(3alpha,8alpha)-3,17-dihydroxypregn-5-en-20-one | C21 H32 O3 | 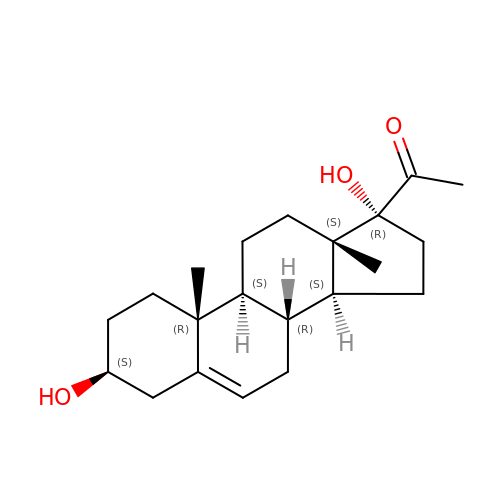JERGUCIJOXJXHF-TVWVXWENSA-N3-[2-[(~{Z})-[5-[(~{Z})-[(4~{R})-3-ethylidene-4-methyl-5-oxidanylidene-pyrrolidin-2-ylidene]methyl]-3-(3-hydroxy-3-oxopropyl)-4-methyl-pyrrol-2-ylidene]methyl]-5-[(~{Z})-(4-ethyl-3-methyl-5-oxidanylidene-pyrrol-2-ylidene)methyl]-4-methyl-1~{H}-pyrrol-3-yl]propanoic acid | 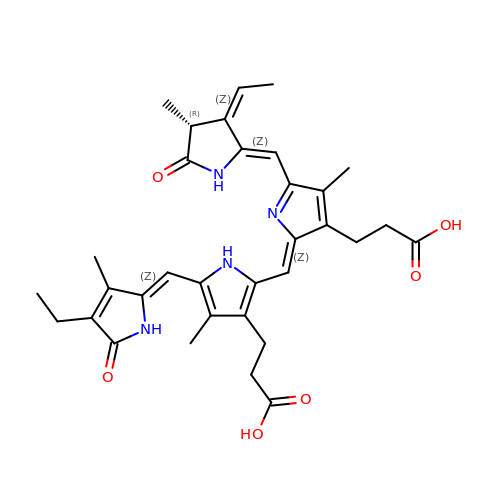C33 H38 N4 O6 | XAVVMXGLKJSJDU-NSNBCYBJSA-N> GGGRMAVQVVQAVQAVHLESDAFLVCLNHALSTEKEEVMGLCIGELNDDIRSDSKFTYTGTEMRTVQEKMDTIRIVHIHSVIILRRSDKRKDRVEISPEQLSAASTEAERLAELTGRPMRVVGWYHSHPHITVWPSHVDVRTQAMYQMMDQGFVGLIFSCFIEDKNTKTGRVLYTCFQSIQAQKSSEYERIEIPIHIVPHITIGKVCLESAVELPKILCQEEQDAYRRIHSLTHLDSVTKIHNGSVFTKNLCSQMSAVSGPLLQW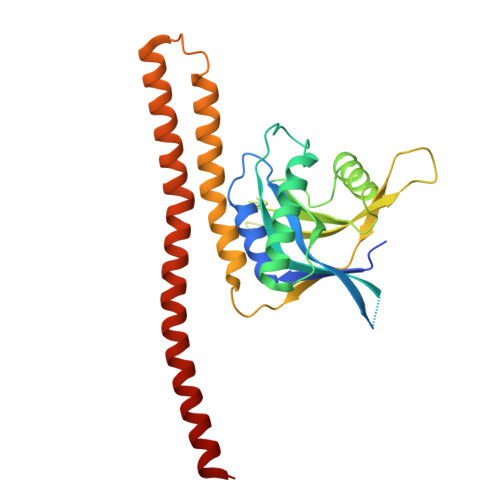LEDRLEQNQQHLQELQQEKEELMEELSSLE>MNSQQNPDLAVHPLAIPMEGLLGESATTLEKNVIATQLSEEAQVKLEVIQSLLEPCDRTTYGQKLREAAEKLNVSLRTVQRLVKNWEQDGLVGLTQTSRADKGKHRIGEFWENFITKTYKEGNKGSKRMTPKQVALRVEAKAR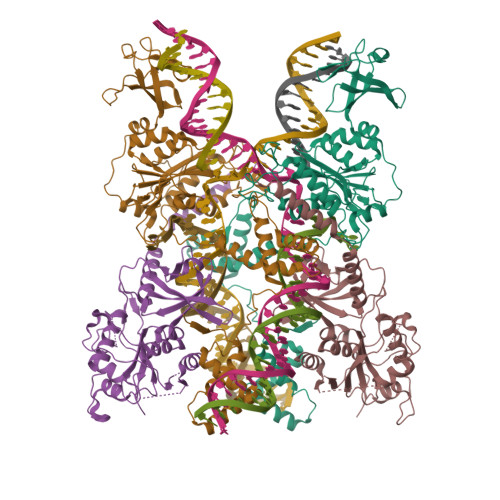ELKDSKPPNYKTVLRVLAPILEKQQKAKSIRSPGWRGTTLSVKTREGKDLSVDYSNHVWQCDHTRVDVLLVDQHGEILSRPWLTTVIDTYSRCIMGINLGFDAPSSGVVALALRHAILPKRYGSEYKLHCEWGTYGKPEHFYTDGGKDFRSNHLSQIGAQLGFVCHLRDRPSEGGVVERPFKTLNDQLFSTLPGYTGSNVQERPEDAEKDARLTLRELEQLLVRYIVDRYNQSIDARMGDQTRFERWEAGLPTVPVPIPERDLDICLMKQSRRTVQRGGCLQFQNLMYRGEYLAGYAGETVNLRFDPRDITTILVYRQENNQEVFLTRAHAQGLETEQLALDEAEAASRRLRTAGKTISNQSLLQEVVDRDALVATKKSRKERQKLEQTVLRSAAVDESNRESLPSQIVEPDEVESTETVHSQYEDIEVWDYEQLREEYGFGSEFELENLYFQ[4x]> GSMGENNMSSIAPHPVVHVALLPSAGMGHLTPFLRLASLLLHQHCHVTLITPQPTVSKAEEDLLSRFLSAFPQVNQLHFHLPPSDSTISTDPFFLQFASIRSSSHLLTPLLSSLTPPLSSFIYDMTLISPLLPIAESLGVPHYILFTSSATMFSFFSYFPTLAKSESFPGKLDFVEIPGVSVSSIPRSSIPPPLLVPNSLFGKLFMEDSPKLKKLHGVLVNT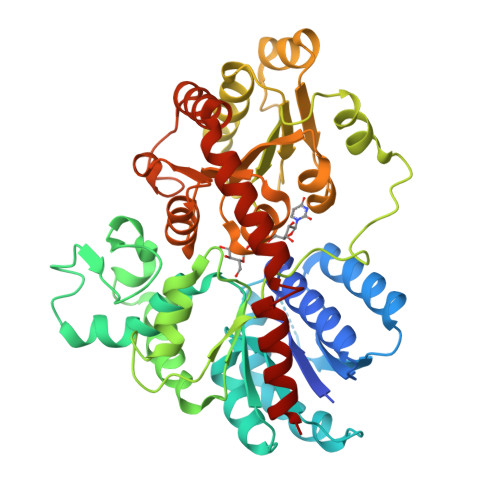FEGIEKLSLEALNGGKVVKGLPPVYGVGPFVPCEFEKVVKRGETISEWLDEQPSGSVVYVSFGSRTAMGREQLREVGDGLVKSGWRFLWVVKDKIVDRAEEEGLDGVLGFELVERMVKEKKGLVVKEWVDQSEILGHKAVGGFVSHCGWNSVVEAAWFGVKILGWPLHGDQKINAEVVAKGGWGVWKEGWDWEGERLVKGEEIGEAIREVMNDESLVMKATQVKKDARKAISVGGGCEVALQKLMEVWKKNV>MTKRVRLSDSFNPVYPYEDESTSQHPFINPGFISPNGFTQSPNGVLTLKCLTPLTTTGGSLQLKVGGGLTVDDTNGFLKENISATTPLVKTGHSIGLPLGAGLGTNENKLCIKLGQGLTFNSNNICIDDNINTLWTGVNPTEANCQIMNSSESNDCKLILTLVKTGALVTAFVYVIGVSNNFNMLTTHRNINFTAELFFDSTGNLLTRLSSLKTPLNHKSGQNMATGAITNAKGFMPSTTAYPFNDNSREKENYIYGTCYYTASDRTAFPIDISVMLNRRAINDETSYCIRITWSWNTGDAPEVQTSATTLV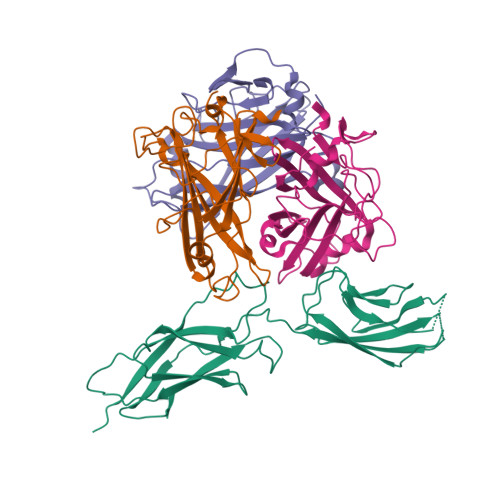TSPFTFYYIREDD[3x];> MARSPGRAYALLLLLICFNVGSGLHLQVLSTRNENKLLPKHPHLVRQKRAWITAPVALREGEDLSKKNPIAKIHSDLAEERGLKITYKYTGKGITEPPFGIFVFNKDTGELNVTSILDREETPFFLLTGYALDARGNNVEKPLELRIKVLDINDNEPVFTQDVFVGSVEELSAAHTLVMKINATDADEPNTLNSKISYRIVSLEPAYPPVFYLNKDTGEIYTTSVTLDREEHSSYTLTVEARDGNGEVTDKPVKQAQVQIRILDVNDNIPVVENKVLEGMVEENQVNVEVTRIKVFDADEIGSDNWLANFTFASGNEGGYFHIETDAQTNEGIVTLIKEVDYEEMKNLDFSVIVANKAAFHKSIRSKYKPTPIPIKVKVKNVKEGIHFKSSVISIYVSESMDRSSKGQIIGNFQAFDEDTGLPAHARYVKLEDRDNWISVDSVTSEIKLAKLPDFESRYVQNGTYTVKIVAISEDYPRKTITGTVLINVEDINDNCPTLIEPVQTICHDAEYVNVTAEDLDGHPNSGPFSFSVIDKPPGMAEKWKIARQESTSVLLQQSEKKLGRSEIQFLISDNQGFSCPEKQVLTLTVCECLHGSGCREAQHDSYVGLGPAAIALMILAFLLLLLVPLLLLMCHCGKGAKGFTPIPGTIEMLHPWNNEGAPPEDKVVPSFLPVDQGGSLVGRNGVGGMAKEATMKGSSSASIVKGQHEMSEMDGRWEEHRSLLSGRATQFTGATGAIMTTETTKTARATGASRDMAGAQAAAVALNEEFLRNYFTDKAASYTEEDENHTAKDCLLVYSQEETESLNASIGCCSFIEGELDDRFLDDLGLKFKTLAEVCLGQKIDINKEIEQRQKPATETSMNTASHSLCEQTMVNSENTYSSGSSFPVPKSLQEANAEKVTQEIVTERSVSSRQAQKVATPLPDPMASRNVIATETSYVTGSTMPPTTVILGPSQPQSLIVTERVYAPASTLVDQPYANEGTVVVTERVIQPHGGGSNPLEGTQHLQDVPYVMVRERESFLAPSSGVQPTLAMPNIAVGQNVTVTERVLAPASTLQSSYQIPTENSMTARNTTVSGAGVPGPLPDFGLEESGHSNSTITTSSTRVTKHSTVQHSYS> QIGWRREGIKYRRNELFLDVLESVNLLMSPQGQVLSAHVSGRVVMKSYLSGMPECKFGMNDKIVIEKQGKGTADETSKSGKQSIAIDDCTFHQCVRLSKFDSERSISFIPPDGEFELMRYRTTKDIILPFRVIPLVREVGRTKLEVKVVIKSNFKPSLLAQKIEVRIPTPLNTSGVQVICMKGKAKYKASENAIVWKIKRMAGMKESQISAEIELLPTNDKKKWARPPISMNFEVPFAPSGLKVRYLKVFEPKLNYSDHDVIKWVRYIGRSGIYETRC;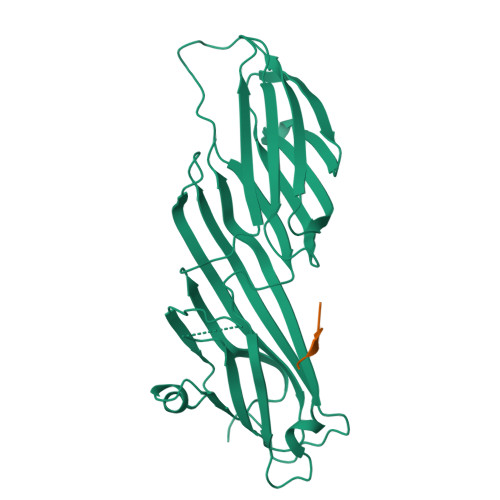> DYMPMSPK>[4x]MDSLDQCIVNACKNSWDKSYLAGTPNKDNCSGFVQSVAAELGVPMPRGNANAMVDGLEQSWTKLAS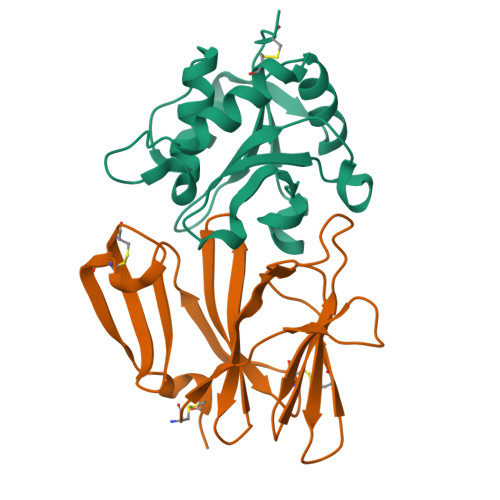GAEAAQKAAQGFLVIAGLKGRTYGHVAVVISGPLYRQKYPMCWCGSIAGAVGQSQGLKSVGQVWNRTDRDRLNYYVYSLASCSLPRASLEHHHHHH;>MADCTFTQLEIVPQFGSPNMFGGEDEHVRVMFSNEDPNDDNPDAFPEPPVYLADRDSGNDCRIEDGGIWSRGGVFLSQDGRRVLMHEFSGSSAELVSYDSATCKVVHREDISGQRWAVDKDGLRLGQKCSGESVDSCAKIVKRSLAPFCQTAKKLEHHHHHH[4x]>MSLQIVPYLIFNGNCREAFSCYHQHLGGTLEAMLPFGDSPECGDIPADWKDKIMHARLVVGSFALMASDNHPAYPYEGIKGCSISLNVDSKAEAERLFNALAEGGSVQMPLGPTFWAASFGMFTDRFGVAW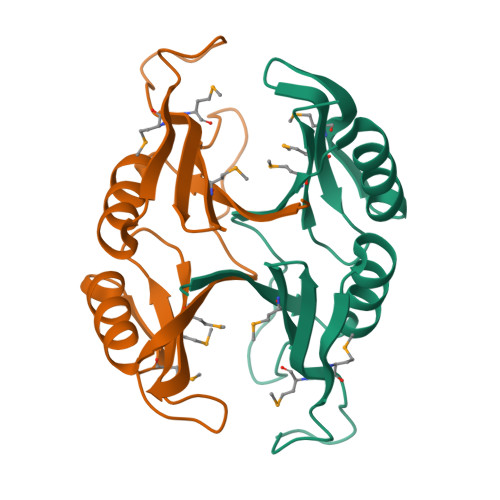MVNCEQDREGGSHHHHHH[2x]[4-(2-hydroxyethyl)piperidin-1-yl][4-(5-methyl-4,4-dioxido-1,5-dihydropyrazolo[4,3-c][2,1]benzothiazin-8-yl)phenyl]methanone 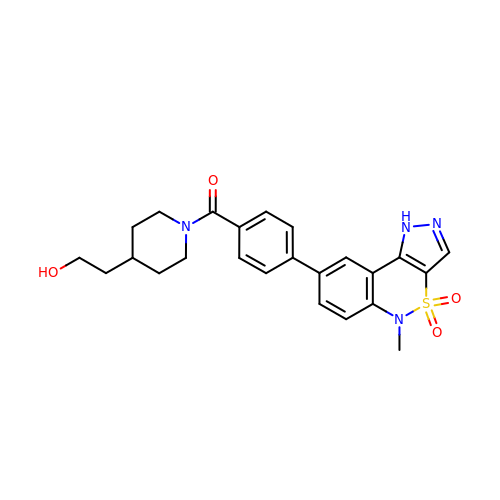| C24 H26 N4 O4 S | FADYFQASOSLUAS-UHFFFAOYSA-N>ASNFEEFVLVDNGGTGDVKVAPSNFANGVAEWISSNSRSQAYKVTCSVRQSSANNRKYTVKVEV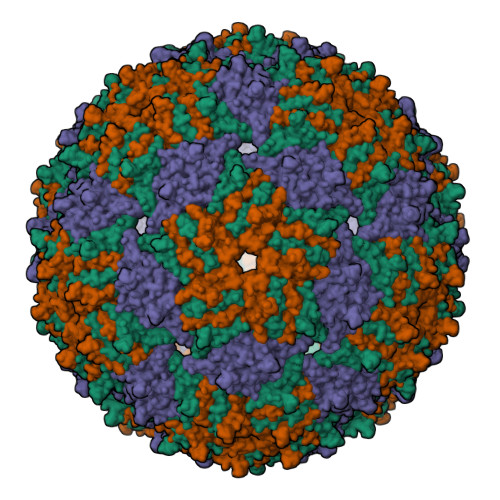PKVATQVQGGVELPVAAWRSYMNMELTIPVFATNDDCALIVKALQGTFKTGNPIATAIAANSGIY[3x]> MEVGQMRRQWVDYIKSMFMEGFLDGQFLQLQQLQDENNPEFVFE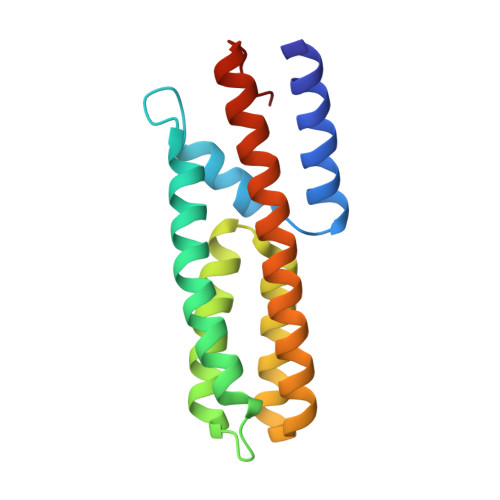VVSLFFDDSERILKDLSFAVDQQSIDFKKVDAHVHQFKGSSASIGAQRVKNSCVAFRNFCEEQNIDACRRCLQQVKQEYLLVKNKLETLLRLEQQIVAAGGSIPMMELN>MIFGHGDEGITPLSSEIVNFSTTVWTDGDKDHLEKHLVENLNCIRHYPEPDAGTLRQMLAKRNSVDNNAILVTNGPTAAFYQIAQAFRGSRSLIAIPSFAEYEDACRMYEHEVCFYPSNEDIGEADFSNMDFCWLCNPNNPDGRLLQRTEILRLLNDHPDTTFVLDQSYVSFTTEEVIRPADIKGRKNLVMVYSFSHAYGIPGLRIGYIVANKDFMKRVAAFSTPWAVNALAIEAAKFILIHPAQFTLPIRKWQRNTVDFITALNRLDGVEVHPSGTTFFLLRLKKGTAAELKKYMLEEYNMLIRDASNFRGLDESYV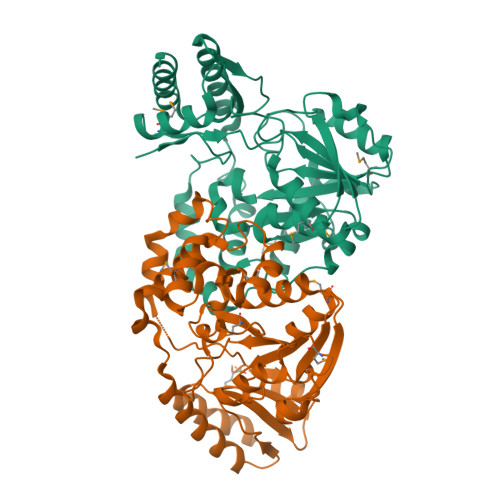RITTQRPAQNQLFIKALETFLEKYEGHHHHHH[4x]>MHHHHHHGLLKESMRIKMDMEGTVNGHYFKCEGEGDGNPFTGTQSMRIHVTEGAPLPFAFDILAPCCXSRTFIHHTAGIPDFFKQSFPEGFTWERTTTYEDGGILTAHQDTSLEGNCLIYKVKVLGTNFPADGPVMKNKSEGWEPCTEVVYPDNGVLCGRNVMALKVGDRR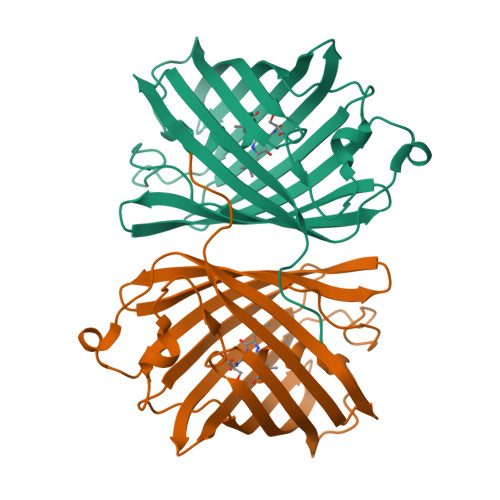LICHLYSSYKSKKAIRALTMPGFHFTDIRLQMPRKKKDEYFELYEASVARYSDLPEK[8x]> GMSQPKKRKLESGGGGEGGEGTEEEDGAEREAALERPRRTKRERDQLYYECYSDVSVHEEMIADRVRTDAYRLGILRNWAALRGKTVLDVGAGTGILSIFCAQAGARRVYAVEASAIWQQAREVVRFNGLEDRVHVLPGPVETVELPEQVDAIVSEWMGYGLLHESMLSSVLHARTKWLKEGGLLLPASAELFIVPISDQMLEWRLGFWS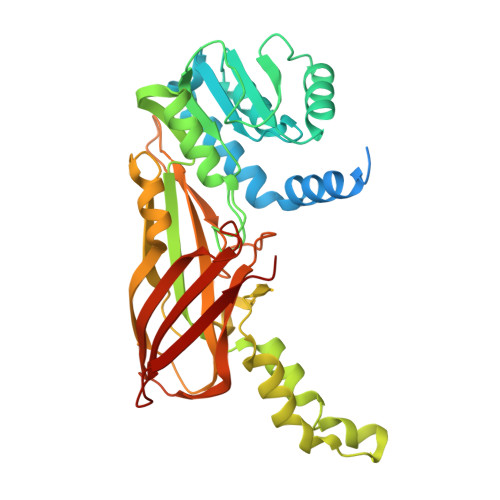QVKQHYGVDMSCLEGFATRCLMGHSEIVVQGLSGEDVLARPQRFAQLELSRAGLEQELEAGVGGRFRCSCYGSAPMHGFAIWFQVTFPGGESEKPLVLSTSPFHPATHWKQALLYLNEPVQVEQDTDVSGEITLLPSRDNPRRLRVLLRYKVGDQEEKTKDFAMED>[4x]MKDLK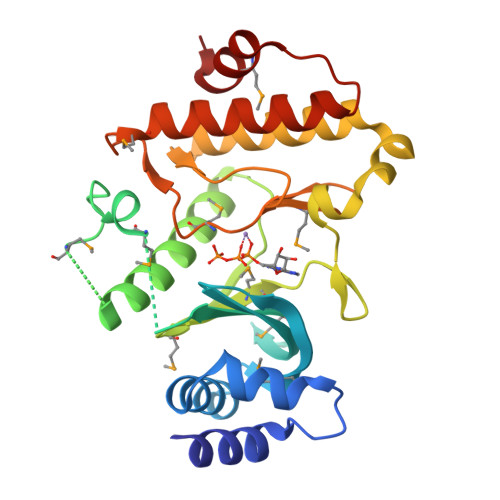KIESYLDKLRIKEKDGEERKIYAEVLDGRTLKTLYKLSAKGYITAMGGVISTGKEANVFYADGVFDGKPVAMAVKIYRIETSEFDKMDEYLYGDERFDMRRISPKEKVFIWTEKEFRNLERAKEAGVSVPQPYTYMKNVLLMEFIGEDELPAPTLVELGRELKELDVEGIFNDVVENVKRLYQEAELVHADLSEYNIMYIDKVYFIDMGQAVTLRHPMAESYLERDVRNIIRFFSKYGVKADFEEMLKEVKGE> STGG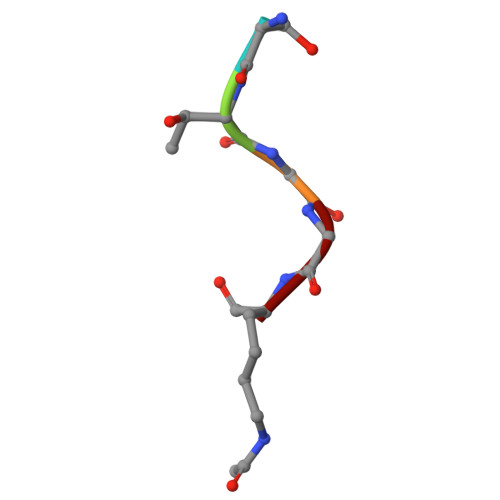K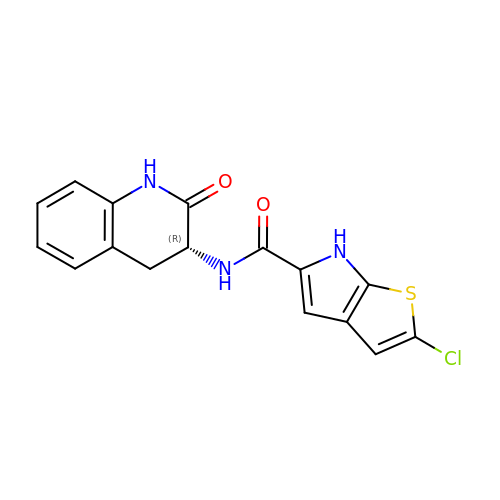2-CHLORO-N-[(3R)-2-OXO-1,2,3,4-TETRAHYDROQUINOLIN-3-YL]-6H-THIENO[2,3-B]PYRROLE-5-CARBOXAMIDE | C16 H12 Cl N3 O2 S | LJAHIGGEXIWVJG-LLVKDONJSA-N> MKRNYILGLDIGITSVGYGIIDYETRDVIDAGVRLFKEANVENNEGRRSKRGARRLKRRRRHRIQRVKKLLFDYNLLTDHSELSGINPYEARVKGLSQKLSEEEFSAALLHLAKRRGVHNVNEVEEDTGNELSTKEQISRNSKALEEKYVAELQLERLKKDGEVRGSINRFKTSDYVKEAKQLLKVQKAYHQLDQSFIDTYIDLLETRRTYYEGPGEGSPFGWKDIKEWYEMLMGHCTYFPEELRSVKYAYNADLYNALNDLNNLVITRDENEKLEYYEKFQIIENVFKQKKKPTLKQIAKEILVNEEDIKGYRVTSTGKPEFTNLKVYHDIKDITARKEIIENAELLDQIAKILTIYQSSEDIQEELTNLNSELTQEEIEQISNLKGYTGTHNLSLKAINLILDELWHTNDNQIAIFNRLKLVPKKVDLSQQKEIPTTLVDDFILSPVVKRSFIQSIKVINAIIKKYGLPNDIIIELAREKNSKDAQKMINEMQKRNRQTNERIEEIIRTTGKENAKYLIEKIKLHDMQEGKCLYSLEAIPLEDLLNNPFNYEVDHIIPRSVSFDNSFNNKVLVKQEEASKKGNRTPFQYLSSSDSKISYETFKKHILNLAKGKGRISKTKKEYLLEERDINRFSVQKDFINRNLVDTRYATRGLMNLLRSYFRVNNLDVKVKSINGGFTSFLRRKWKFKKERNKGYKHHAEDALIIANADFIFKEWKKLDKAKKVMENQMFEEKQAESMPEIETEQEYKEI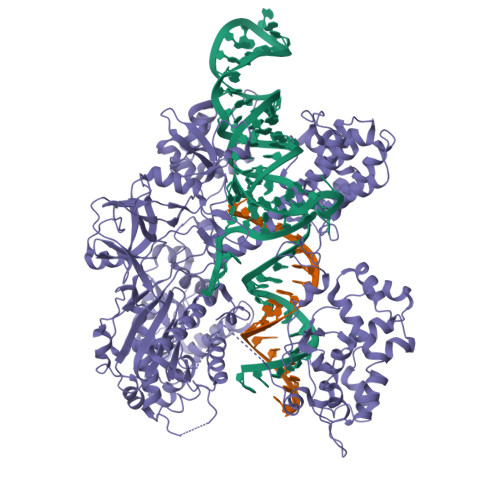FITPHQIKHIKDFKDYKYSHRVDKKPNRELINDTLYSTRKDDKGNTLIVNNLNGLYDKDNDKLKKLINKSPEKLLMYHHDPQTYQKLKLIMEQYGDEKNPLYKYYEETGNYLTKYSKKDNGPVIKKIKYYGNKLNAHLDITDDYPNSRNKVVKLSLKPYRFDVYLDNGVYKFVTVKNLDVIKKENYYEVNSKAYEEAKKLKKISNQAEFIASFYNNDLIKINGELYRVIGVNNDLLNRIEVNMIDITYREYLENMNDKRPPRIIKTIASKTQSIKKYSTDILGNLYEVKSKKHPQIIKKG>[4x]MGSSHHHHHHSSENLYFQGHMSDLPRISVAAPRLDGNERDYVLECMDTTWISSVGRFIVEFEKAFADYCGVKHAIACNNGTTALHLALVAMGIGPGDEVIVPSLTYIASANSVTYCGATPVLVDNDPRTFNLDAAKLEALITPRTKAIMPVHLYGQICDMDPILEVARRHNLLVIEDA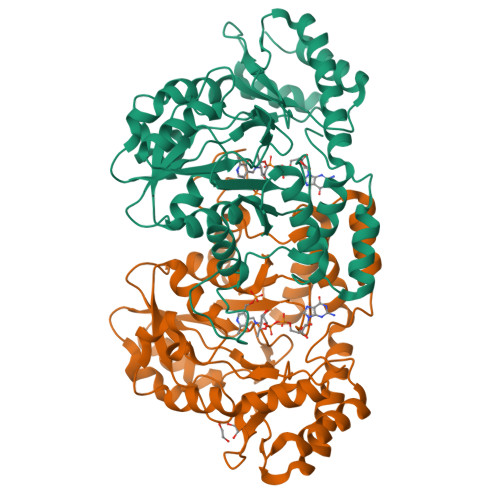AEAVGATYRGKKSGSLGDCATFSFFGNAIITTGEGGMITTNDDDLAAKMRLLRGQGMDPNRRYWFPIVGFNYRMTNIQAAIGLAQLERVDEHLAARERVVGWYEQKLARLGNRVTKPHVALTGRHVFWMYTVRLGEGLSTTRDQVIKDLDALGIESRPVFHPMHIMPPYAHLATDDLKIAEACGVDGLNLPTHAGLTEADIDRVIAALDQVLV>[6x]AQQMPSLAPMLEKVMPSVVSINVEGSTTVNTPRMPRNFQQFFGDDSPFCQEGSPFQSSPFCQGGQGGNGGGQQQKFMALGSGVIIDADKGYVVTNNHVVDNATVIKVQLSDGRKFDAKMVGKDPRSDIALIQIQNPKNLTAIKMADSDALRVGDYTVAIGNPFGLGETVTSGIVSALGRSGLNAENYENFIQTDAAINRGNAGGALVNLNGELIGINTAILAPDGGNIGIGFAIPSNMVKNLTSQMVEYGQVKRGELGIMGTELNSELAKAMKVDAQRGAFVSQVLPNSSAAKAGIKAGDVITSLNGKPISSFAALRAQVGTMPVGSKLTLGLLRDGKQVNVNLELQQSSQNQVDSSSIFNGIEGAEMSNKGKDQGVVVNNVKTGTPAAQIGLKKGDVIIGANQQAVKNIAELRKVLDSKPSVLALNIQRGDSTIYLLMQ;>CYYKI[12x]

First, DegP is an allosteric protease, whose activity is carefully regulated, and a hyperactive DegP variant kills bacteria. Second, because DegP is an inherently promiscuous protease that degrades misfolded proteins, over-activated DegP may destroy various proteins that mediate essential processes in the bacterial envelope, such as cell wall maintenance, membrane construction, or cell division. Previous report showed that substrate binding accompanies several allosteric behaviors of DegP: proteolytic activation, assembly of cage-like proteolytic chamber and positively cooperative binding of a substrate. DegP mainly degrades misfolded proteins, but its over-activation by the tripodal compounds triggers excessive degradation of newly synthesized proteins and leads to bacterial death.

We also tested the tripodal compound with the CYYKI arms (TMB_CYYKI). As expected, we obtained a similar biphasic curve with the maximal activation at around 10 µM, suggesting that this compound interacts with DegP more tightly than TMB_CYRKL (black circle). Alanine scanning of the peptide showed that the C-terminal isoleucine and two tyrosines are critical for the activation and tight binding of DegP. Denatured OmpA was degraded not by DegP alone, but by TMB_CYYKI-activated DegP, indicating that the compound induces degradation of a protein that is not efficiently recognized and degraded by DegP. By contrast, TMB_CYYKI functions as a permanent activator; it remained almost intact and still activated DegP after longer incubation times (1–4 h) with DegP. Overall DegP structures were almost identical to that of the dodecameric DegP with an active conformation (rmsd 0.697 Å and 0.986 Å, respectively, for 2309 Cα atoms in six DegP subunits). Additional electron density maps were found at positions where two degrons of 18–58 are present in the dodecamer model. Because CYRKL and CYYKI have hydrophobic C-terminal residues that can occupy both the S1 pocket of the active site and the hydrophobic pocket of PDZ1, we believe that these peptides are located in the two substrate-binding sites in the same fashion as two degrons of 18–58. Although the lack of electron density for the central benzene ring hampers determination of the binding mode, we suggest that only one arm of the tripodal compounds in the co-crystal structures binds to either substrate-binding sites of DegP, because the distances between two cysteine-Cα atoms in the CYYKI peptides of the crystal structure are too long to justify any of the three plausible modes for the bi- or tri-partite interactions. Taken together, the crystal structures suggest that the tripodal compounds mainly bind to the substrate-binding sites of DegP.> IDYPSVSFNLAGAKSTTYRDFLKNLRDRVATGTYEVNGLPVLRRESEVQVKNRFVLVRLTNYNGDTVTSAVDVTNLYLVAFSANGNSYFFKDATELQKSNLFLGTTQHTLSFTGNYDNLETAAGTRRESIELGPNPLDGAITSLWYDGGVARSLLVLIQMVPEAARFRYIEQEVRRSLQQLTSFTPNALMLSMENNWSSMSLEVQLSGDN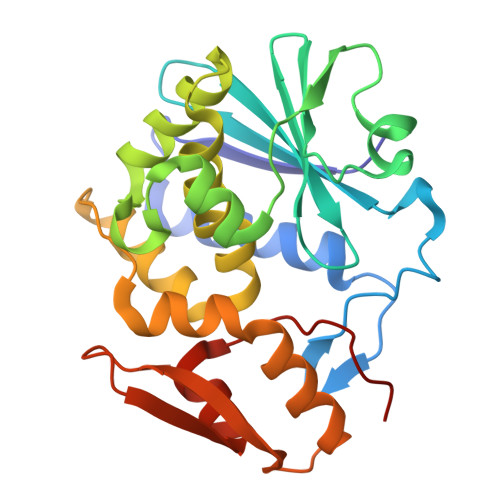VSPFSGTVQLQNYDHTPRLVDNFEELYKITGIAILLFRCVATKT>[2x]MTTGVRRRMGVEERRQQLIG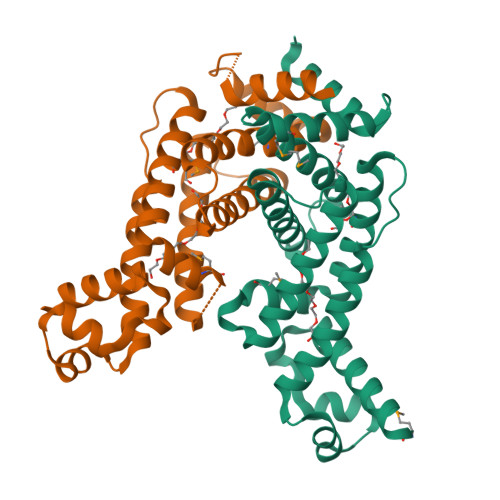VALDLFSRRSPDEVSIDEIASAAGISRPLVYHYFPGKLSLYEAALQRASDDLADRFVEPRQGPLGARLLRVMGRYFDFVDEHGPGFSALMRGGPAVGSTTTNALVDSVRQAAYVQILSHLDVTEPPARLELVVRSWISLAESTALLWLDGRRIPRAELETQLVHDFAALMAVSAAYDEEMGALVRRVLADEPEDGPFGDLVDRLLALSARG> KEFNNPINFQDTETRYGGIQNQVVNINQYVQRNPNFIDLDNIAELSEHSVNTERVKTGDRGMSHKEGGWPGNVDPNEAQETGRFKKRIEKDTSFPQAVKDLKEGVEKCIYQNNQIDLLEEYFEGETSEHVVENLSSKTLMLFKDEKEICKRSVSEISWHPEGPTKVAVSYAIMRFQQMPEKMP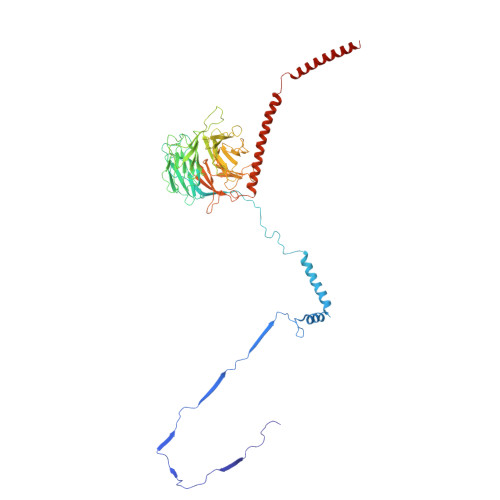TQAYVWDLLNPNSPEIKLMSPSAVTNISYNQKIPDQIGGGCYNGLLAVWDGRKGENPIMISPVENSHYEPVTHFHWLMSKTGSECVTTSTDGKVMWWDTRKFEAGPVEKLNIIEGLGENEEIIGGTALEYNVEAGPSKFLIGTESGSILTANKKLKKPVEITTRYGLDQGRHLGPVYSINRSNQNPKYFLSVGDWSCKIWVEDLKTPIIRTKYHGSYLSDGCWSPTRSGAFFLVRRDGWMDVWDYYYRQNEIAFSHKVSDSPLTCIKINQTGGAYHNSGKLCAIGDQDGTVTILELCDSLYTMQPKEKDIINEMFEREYRKEKNLETIKKQQELAKRQVQKDMGSQKEKWEKKKLEMIETAEASFHENLAKNPV> MRSMSELIVSRQQRVLLLTLNRPAARNALNNALLMQLVNELEAAATDTSISVCVITGNARFFAAGADLNEMAEKDLAATLNDTRPQLWARLQAFNKPLIAAVNGYALGAGCELALLCDVVVAGENARFGLPEITLGIMPGAGGTQRLIRSVGKSLASKMVLSGESITAQQA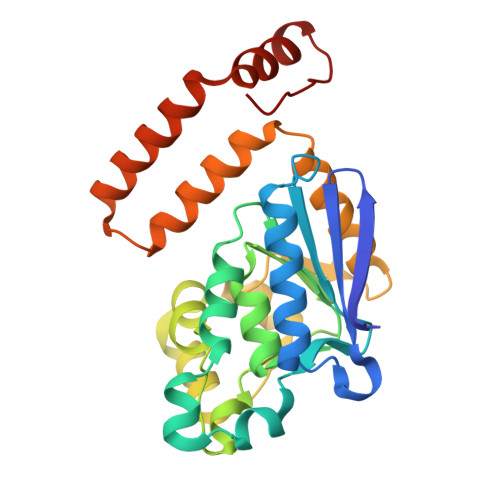QQAGLVSDVFPSDLTLEYALQLASKMARHSPLALQAAKQALRQSQEVALQAGLAQERQLFTLLAATEDRHEGISAFLQKRTPDFKGR>MNGERIIAFQGRPGAYSDLACRQARPGWTTLPCQTFAQTIAAVHDGRAELAM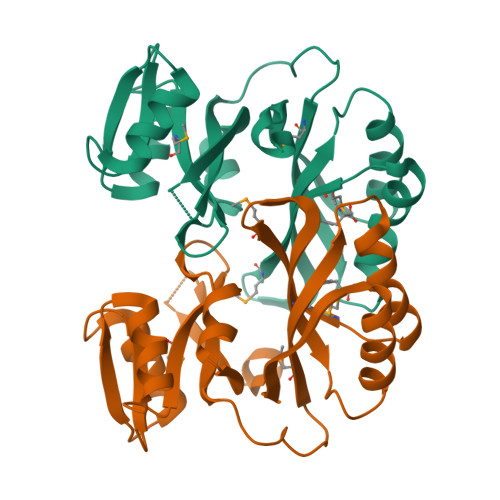LACENSLAGRVPDIHALLPEAGLFIVGEHFQRVEHCLLGIPGSTLADARRIHTHPVAMAQVRGIITELGLDPVVEFDTAGAAEMVREWGRKEDVAVASALAAELNGLEILRRNVEDATHNTTRFYIASRRPATLPPPGPGFMTTLLFRVNNQPGALYKALGGLATAGVNMTRLESYMLEGSFSATQFLMDVEGHPEAPPLARALDELSFFSEQQEILGVYPASPFRRKP[2x]5'-O-[(pyridine-3-carbonyl)sulfamoyl]adenosine | C16 H17 N7 O7 S | 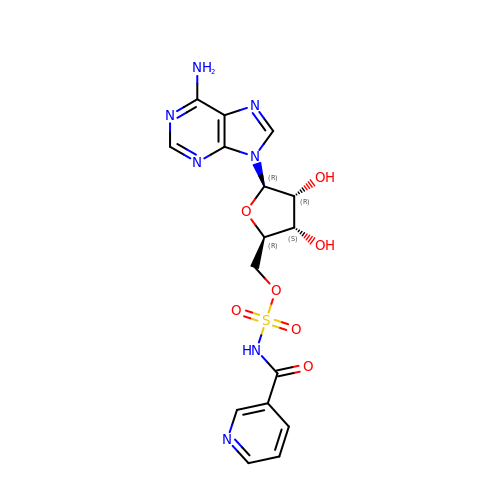LBBNJCOHYSTAJW-UBEDBUPSSA-N>MGQGDESERIVINVGGTRHQTHRSTLRTLPGTRLAWLAEPDAHSHFDYDPRADEFFFDRHPGVFAHILNYYRTGKLHCPADVCGPLYEEELAFWGIDETDVEPCCWMTYRQHRDAEEALDSFGGAPLDNSADDADADGPGDSGDGEDELEMTKRLALSD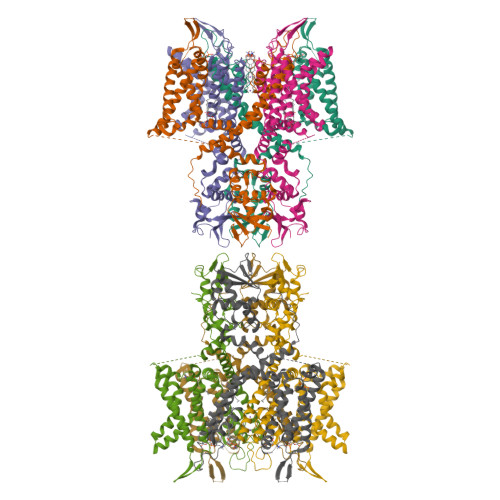SPDGRPGGFWRRWQPRIWALFEDPYSSRYARYVAFASLFFILVSITTFCLETHERFNPIVNKTEIENVRNGTQVRYYREAETEAFLTYIEGVCVVWFTFEFLMRVIFCPNKVEFIKNSLNIIDFVAILPFYLEVGLSGLSSKAAKDVLGFLRVVRFVRILRIFKLTRHFVGLRVLGHTLRASTNEFLLLIIFLALGVLIFATMIYYAERIGAQPNDPSASEHTHFKNIPIGFWWAVVTMTTLGYGDMYPQTWSGMLVGALCALAGVLTIAMPVPVIVNNFGMYYSLAMAKQKLPKKKKKHIPRPPQLGSPNYCKSVVNSPHHSTQSDTCPLAQEEILEINRAGRKPLRGMSIAENLYFQ[8x]> GPYMIQEEEWDRDLLLDPAWEKQQRKTFTAWCNSHLRKAGTQIENIEEDFRNGLKLMLLLEVISGERLPKPDRGKMRFHKIANVNKALDYIASKGVKLVSIGAEEIVDGNVKMTLGMIWTIILRFAIQDISVEETSAKEGLLLWCQRKTAPYRNVNIQNFHTSWKDGLGLCALIHRHRPDLIDYSKLNKDDPIGNINLAMEIAEKHLDIPKMLDAEDIVNTPKPDERAIMTYVSCFYHAFAGAEQAETAANRIC;> SEN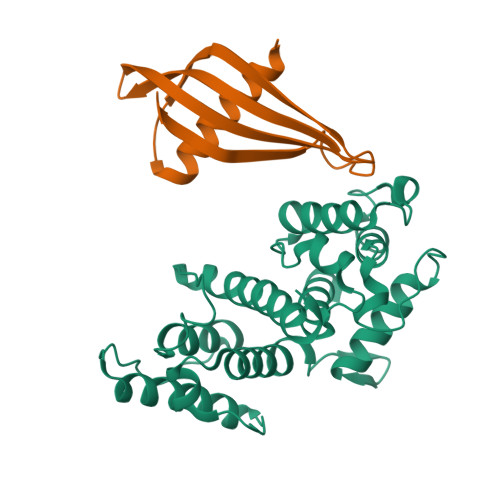SLEIEELARFAVDEHNKKENALLEFVRVVKAKEQHQFHMSWTWTMYYLTLEAKDGGKKKLYEAKVWVKHHPAYIADINFKELQEFKPV> MILDINDVLGKKIITTRLMSSITIHEENSIAALEVMSRFAADPHWLIYLPPTMSPCETSKKEGMLEHPIEAFEYFRTRGVGKVVCEQKHMGSRAVVIVCKDSQVAEKRFGVLDGTAGICYTRTGRHFFDDMQLEAELIDRVRKVLDKSGFWGDFNTDWVCLDCELMPWSAKAQKLLEEQYSAVGISGRVVLDEAVKLLKQASLNKTVSFDVSRQTSGKNADIN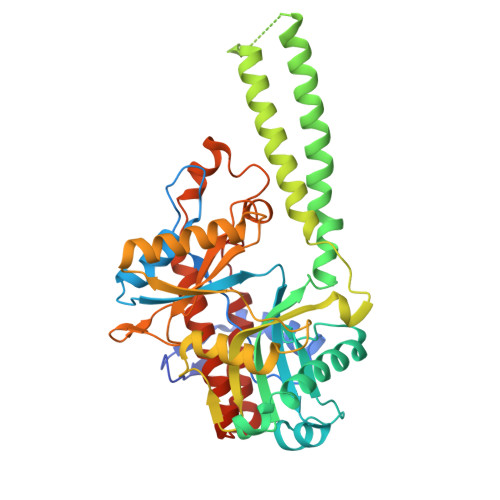ELLQRFTERSEMMQKYVEAYRKYCWPVNSIDDLKLAPFHILATEGKVHSDKNHIWHMDTIAKYCTQDDSLIMATNHILVDVTDAESVDKGIKWWEDLTASGGEGMVVKPYDFIVKNGRELLQPAVKCRGREYLRIIYGPEYTMDENIERLRNRAVGKKRSLALREFSLGMEALERFVRNEPLYRVHECVFGVLALESEPVDPRL>[4x]PRHVRIKNWGSGMTFQDTLHHKAKGILTCRSKSCLGSIMTPKSLTRGPRDKPTPPDELLPQAIEFVNQYYGSFKEAKIEEHLARVEAVTKEIETTGTYQLTGDELIFATKQAWRNAPRCIGRIQWSNLQVFDARSCSTAREMFEHICRHVRYSTNNGNIRSAITVFPQRSDGKHDFRVWNAQLIRYAGYQMPDGSIRGDPANV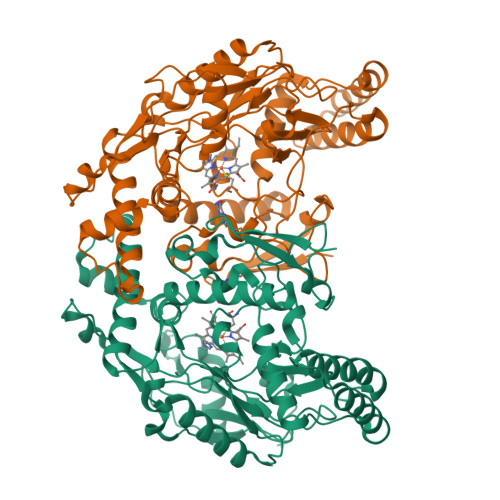EITQLCIDLGWKPKYGRFDVLPLVLQANGRDPELFEIPPDLVLEVAMEHPKYEWFRELELKWYALPAVANMLLEVGGLEFPGCPFNGWYMGTEIGVRDFCDVQRYNILEEVGRRMGLETHKLASLWKDQAVVEINIAVLHSFQKQNVTIMDHHSAAESFMKYMQNEYRSRGGCPADWIWLVPPMSGSITPVFHQEMLNYVLSPFYYYQVEAWKTHVWQDEK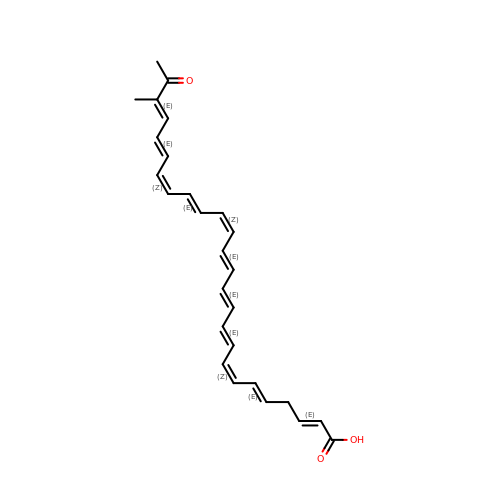(2E,5E,7Z,9E,11E,13E,15Z,17E,19Z,21E,23E)-24-methyl-25-oxohexacosa-2,5,7,9,11,13,15,17,19,21,23-undecaenoic acid | C27 H30 O3 | ZUWHINCAQDXMJU-JXLQPSFDSA-N> MAPKAVLVGLPGSGKSTIGRRLAKALGVGLLDTDVAIEQRTGRSIADIFATDGEQEFRRIEEDVVRAALADHDGVLSLGGGAVTSPGVRAALAGHTVVYLEISAAEGVRRT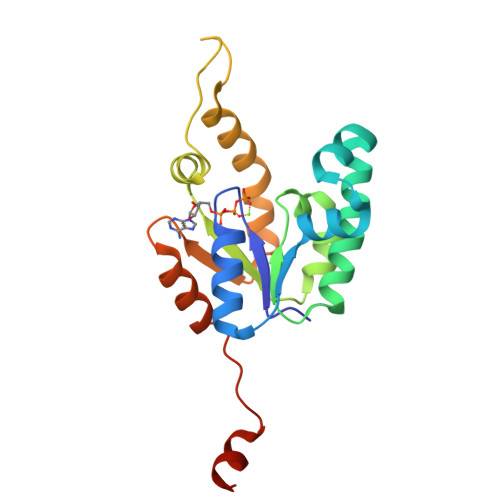GGNTVRPLLAGPDRAEKYRALMAKRAPLYRRVATMRVDTNRRNPGAVVRHILSRLQVPSPSEAATLEHHHHHH> GGRENLYFQGMAEVLMYGLSTCPHCKRTLEFLKREGVDFEVIWIDKLEGEERKKVIEKVHSISGSYSVPVVVKGDKH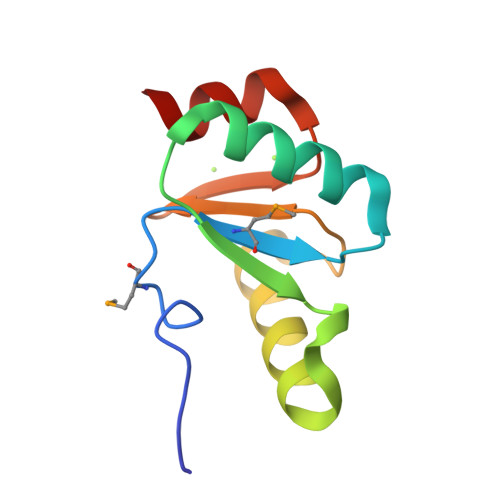VLGYNEEKLKELIRG> SNASKMSDVKCTSVVLLSVLQQLRVESSSKLWAQCVQLHNDILLAKDTTEAFEKMVSLLSVLLSMQGAVDINKLCEEMLDNRATLQ;> EDKRAKVTSAMQTMLFTMLRKLDNDALNNIINNARDGCVPLNIIPLTTAAKLMVVIPDYNTYKNTCDGTTFTYASALWEIQQVVDADSKIVQLSEISMDNSPNLAWPLIVTA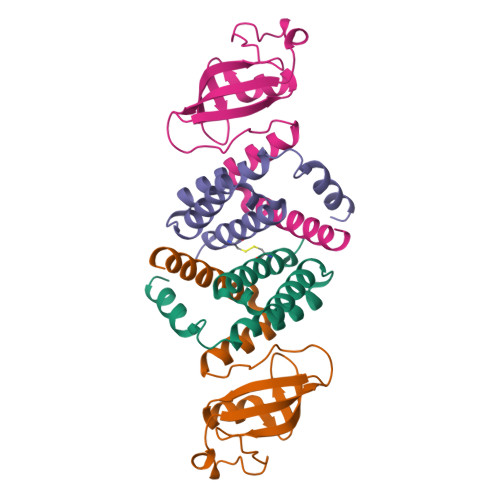LRANSAVKLQ>XLAATLA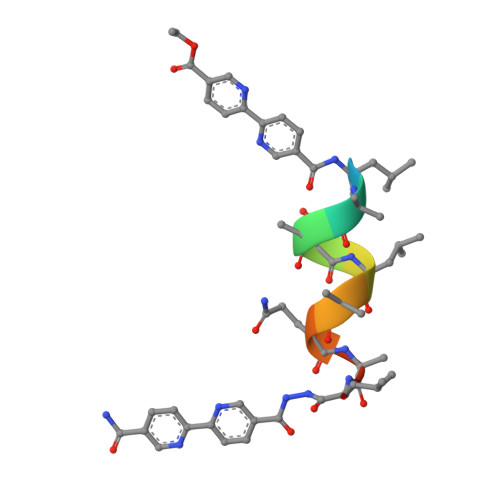QALX[2x]>SNAMNALAATNRNFKLAARLLGLDSKLEKSLLIPFREIKVECTIPKDDGTLASFVGFRVQHDNARGPMKGGIRYHPEVDPDEVNALAQLMTWKTAVAKIPYGGAKGGIGCDPSKLSISELERLTRVFTQKIHDLIGIHTDVPAPDMGTGPQTMAWILDEYSKFHGYSPAVVTGKPIDLGGSLGRDAATGRGVMFGTEALLNEHGKTISGQRFVIQGFGNVGSWAAKLISEKGGKIVAVSDITGAIKNKDGIDIPALLKHTKEHRGVKGFDGADPIDPNSILVEDCDILVPAALGGVINRENANEIKAKFIIEAANHPTDPDADEILSKKGVVILPDIYANSGGVTVSYFEWVQNIQGFMWEEEKVNDELKTYMTRSFK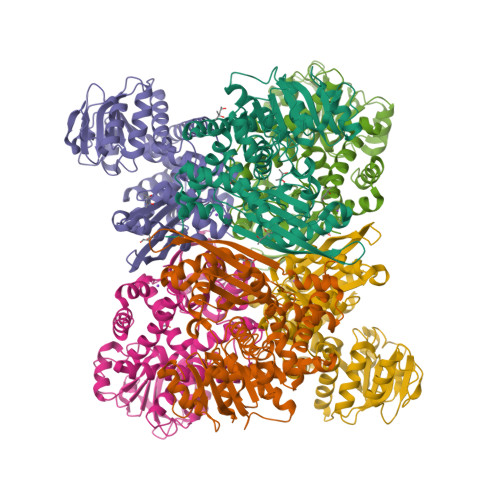DLKEMCKTHSCDLRMGAFTLGVNRVAQATILRGWGA[6x]> MHHHHHHSQDSCISMRQSGCLPLLIQLLHGNDKDSVLLGNSRGSKEARARASAALHNIIHSQPDDKRGRREIRVLHLLEQIRAYCETCWEWQEAHEQGMDQDKNPMPAPVEHQICPAVCVLMKLSFDEEHRHAMNELGGLQAIAELLQVDCEMYGLTNDHY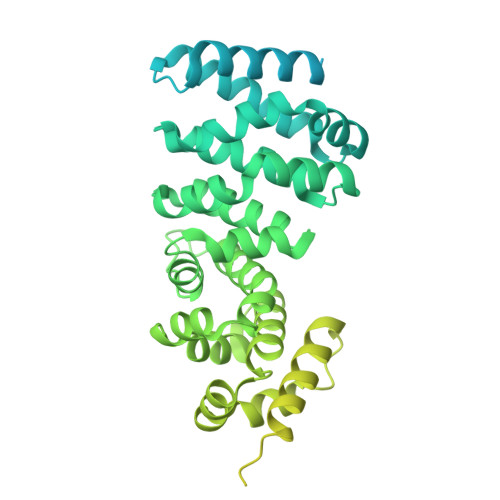SVTLRRYAGMALTNLTFGDVANKATLCSMKGCMRALVAQLKSESEDLQQVIASVLRNLSWRADVNSKKTLREVGSVKALMECALEVKKESTLKSVLSALWNLSAHCTENKADICAVDGALAFLVGTLTYRSQTNTLAIIESGGGILRNVSSLIATNEDHRQILRENNCLQTLLQHLKSHSLTIVSNACGTLWNLSARNPKDQEALWDMGAVSMLKNLIHSKHKMIAMGSAAALRNLMANRPAKYKDANIMSPGSSLPSLHVRKQKALEAELDAQHLSETFDNIDNLSPKASHRSKQRHKQNLYGDYAFDANRHDDSRSDNFNTGNMTVLSPYLNTTVLPSSSSSRGSLDSSRSEKDRSLERERGIGLSAYHPTTENAGTSSKRGLQITTTAAQIAKVMEEVSAIHTSQDDRSSASTTEFHCVADDRSAARRSSASHTHSNTYNFTKSENSNRTCSMPYAKVEYKRSSNDSLNSVTSSDGYGKRGQMKPSVESYSEDDESKFCSYGQYPADLAHKIHSAN>[2x]MSLE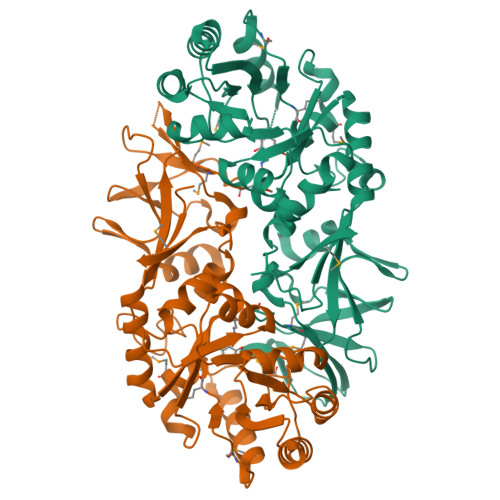AIHRSTRIEFSKSSLAYNVQYTKQVSGAKTLWLAVKSNAYGHGLLQVSKIARECGVDGLAVSVLDEGIAIRQAGIDDFILILGPIDVKYAPIASKYHFLTTVSSLDWLKSADKILGKEKLSVNLAVDTGMNRIGVRSKKDLKDEIEFLQEHSDHFSYDGIFTHFASSDNPDDHYFQRQKNRWYELIDGLIMPRYVHVMNSGAAMYHSKELPGCNSIARVGTVVYGVEPSEGVLGPIDKLKPVFELKSALTFVKKIPAGEGISYGSKFVTSRDTWIGTLPIGYGDGWLAEYQDFQLLIDGQKCRQVGQIAMDQMMVALPHEYPIGTEVTLIGKSGKYENTLYDLHKHSGVPPWKITVAFSDRLKRMVVDEGHHHHHH> ETAAAKFERQHMDSSTSAASSSNYCNQMMKSRNLTKDRCKPVNTFVHESLADVQAVCSQKNVACKNGQTNCYQSYSTMSITDC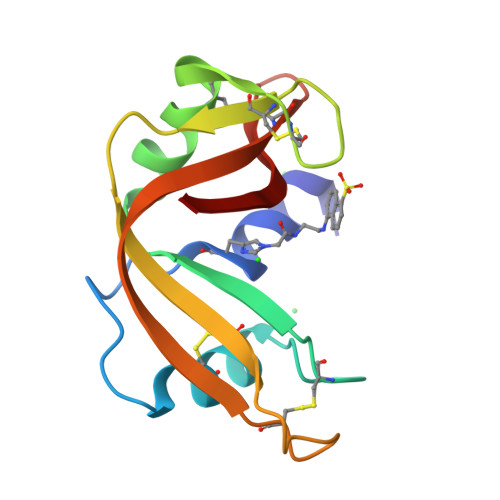RETGSSKYPNCAYKTTQANKHIIVACEGNPYVPVHFDASV>[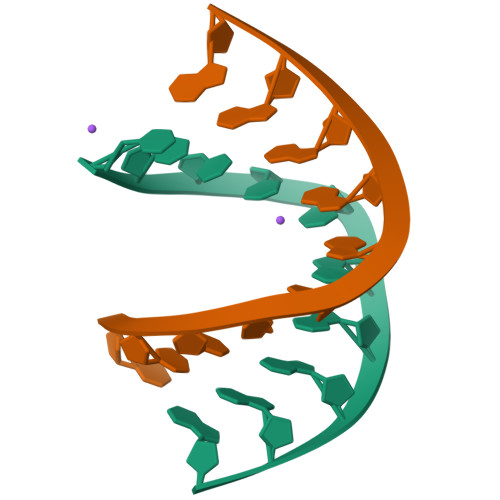2x]CCCCCGGGGG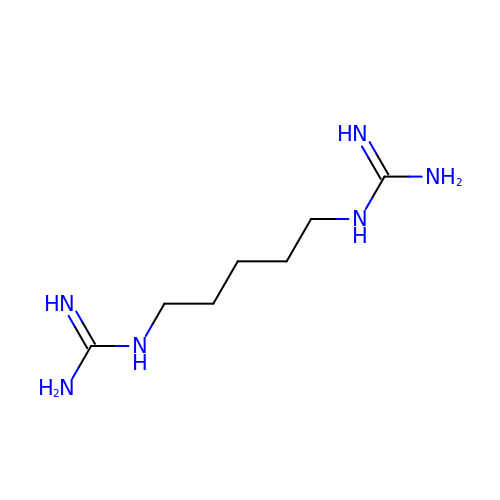1-(5-carbamimidamidopentyl)guanidine | C7 H18 N6 | FIHKQNOFFQZHRM-UHFFFAOYSA-N> GHMRLELPVIPLRNTVILPHTTTPVDVGRAKSKRAVEEAMGADRLIFLVAQRDPEVDDPAPDDLYTWGVQAVVKQAMRLPDGTLQVMVEARARAQVTDYIPGPYLRARGEVFSEIFPIDEAVVRVLVEELKEAFEKYVANHKSLRLDRYQLEAVKGTSDPAMLADTIAYHATWTVAEKQEILELTDLEARLKKVLGLLSRDLERFELDKRVAQRVKEQMDTNQREYYLREQMKAIQKELGGEDGLSDLEALRKKIEEVGMPEAVKTKALKELDR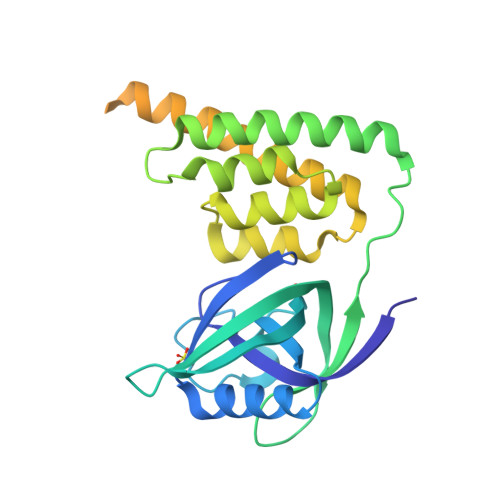LERMQQGSPEATVARTYLD ACETYLSULFATE | C2 H4 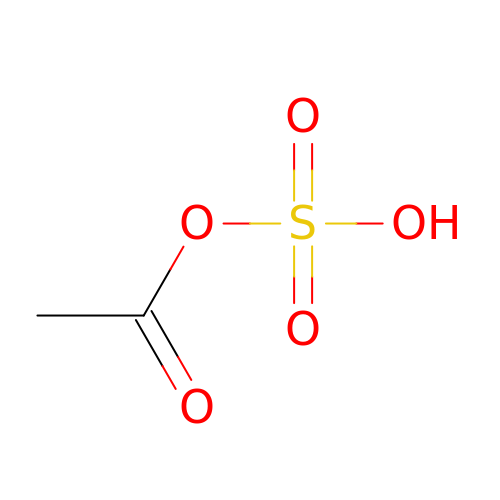O5 S | HZWXJJCSDBQVLF-UHFFFAOYSA-N> SGIALSRLAQERKAWRKDHPFGFVAVPTKNPDGTMNLMNWECAIPGAAGTPWAGGLFKLRMLFKDDYPSSPPKCKFEPPLFHPNVYPSGTVCLSILEEDKDWRPAITIKQI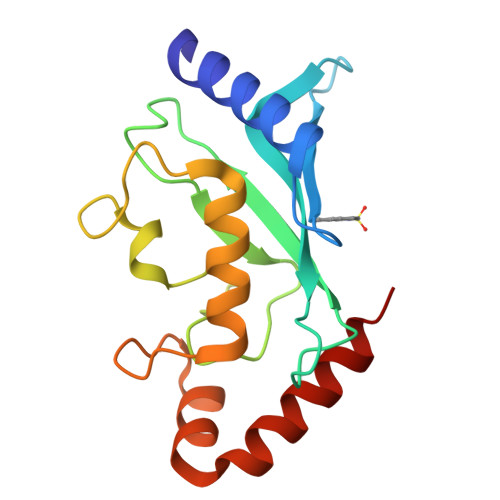LLGIQELLNEPNIQDPAQAEAYTIYCQNRVEYEKRVRAQAKKFAPS> SMKAQSIIERLAAGQVHVYPRSRHESEGTRVQMIKAEGRKYLVAEGSGKLYDELRGEEADGVKLCELSHENRLVLNRHFPFTVPQAFGKQSATIGLGDRLGIAGPGHVQTVRGRAIHPILAQQSIRELALTGRDYKQVIDAAAYAVFQEGYTEGYGADGDHLKKEEDIRMALDLGFTMLTLDCSEQIDNEAAQAGESEVKRKYEELPESVRSHYEAKYLDKTFQVGPHAIHFDAATLMRDVLVYREAIQFMIYIYEKYIQTAGRAVDFEISIDETLTPTAPGSHFLVASELIGKNVDIFSMAPRFIGEFQKGIDYIGDIAQ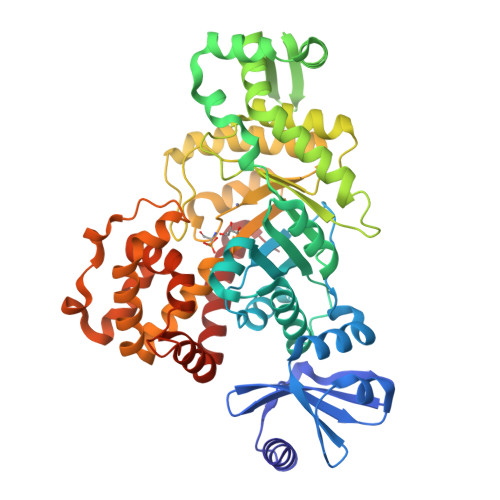FERELAVHAAIADRFGYKLSIHSGSDKFSVFALVGRYTNGRFHVKTAGTNWLEAVRIVAKTNPGLYRRMHQYALEHFEEATAYYHVTTNLNNIRPLADVSDEELPSYMNENDARQLLHITYGLLLQAKKDDGSSLFRDEFFRTLSEREEDYEAALRSHIGKHLDLLGVK>MTQVLVRNGIQAVGDGLTSLIIVGKKSVLKNVTFEGKFKEVAQKFVTDGDSWNSMISRIPASGRHPLHYELAHLITVPDASSRGNTPTNAHSIYKELKPINYPEDTKNVHFVLFAEYPDVLSHVAAIARTFCKFSMKTSGIRELNVNIDVVCDKLTNEDAVFLTDLSESVRETARLIDTPANILTTDALVDEAVKVGNATGSKITVIRGEELLKAGFGGIYHVGKAGPTPPAFVVLSHEVPGSTEHIALVGKGVVYDTGGLQIKTKTGMPNMKRDMGGAAGMLEAYSALVKHGFSQTLHACLCIVE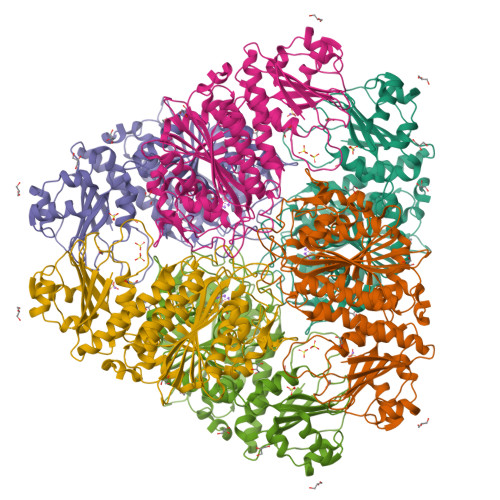NNVSPIANKPDDIIKMLSGKTVEINNTDAEGRLILADGVFYAKETLKATTIFDMATLTGAQAWLSGRLHGAAMTNDEQLENEIIKAGKASGDLVAPMLFAPDLFFGDLKSSIADMKNSNLGKMDGPPSAVAGLLIGAHIGFGEGLRWLHLDIAAPAEVGDRGTGYGPALFSTLLGKYTSVPMLKQ[2x]> VPAFLSKLWTLVEETHTNEFITWSQNGQSFLVLDEQRFAKEILPKYFKHNNMASFVRQLNM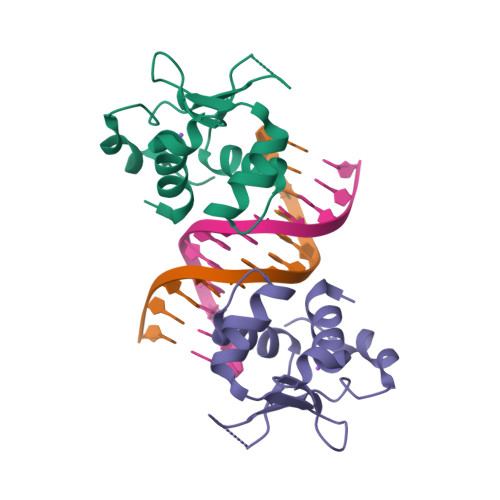YGFRKVVHIDSGIVKQERNGPVEFQHPYFKQGQDDLLENIKRK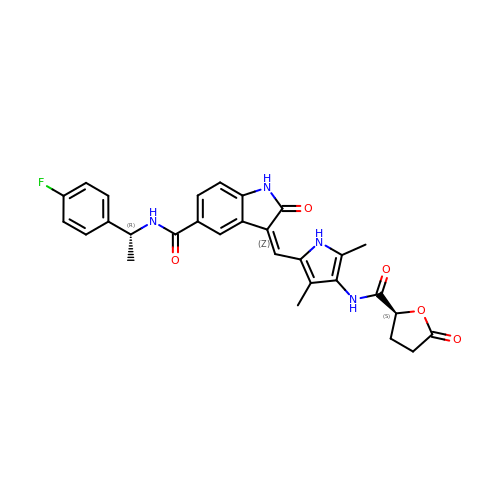(3Z)-3-[(3,5-dimethyl-4-{[(2S)-5-oxooxolane-2-carbonyl]amino}-1H-pyrrol-2-yl)methylidene]-N-[(1R)-1-(4-fluorophenyl)ethyl]-2-oxo-2,3-dihydro-1H-indole-5-carboxamide | C29 H27 F N4 O5 | AWKFMJSRWRFQIH-RUGWSOBISA-N> MWQQAIGDALGITARNLKKFGDRFPHVSDGSNKYVLNDNTDWTDGFWSGILWLCYEYTGDEQYREGAVRTVASFRERLDRFENLDHHDIGFLYSLSAKAQWIVEKDESARKLALDAADVLMRRWRADAGIIQAWGPKGDPENGGRIIIDCLLNLPLLLWAGEQTGD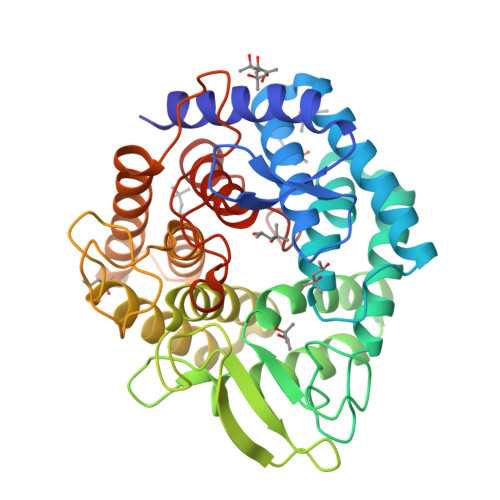PEYRRVAEAHALKSRRFLVRGDDSSYHTFYFDPENGNAIRGGTHQGNTDGSTWTRGQAWGIYGFALNSRYLGNADLLETAKRMARHFLARVPEDGVVYWDFEVPQEPSSYRDSSASAITACGLLEIASQLDESDPERQRFIDAAKTTVTALRDGYAERDDGEAEGFIRRGSYHVRGGISPDDYTIWGDYYYLEALLRLERGVTGYWYERGR> MDETGKELVLALYDYQEKSPREVTM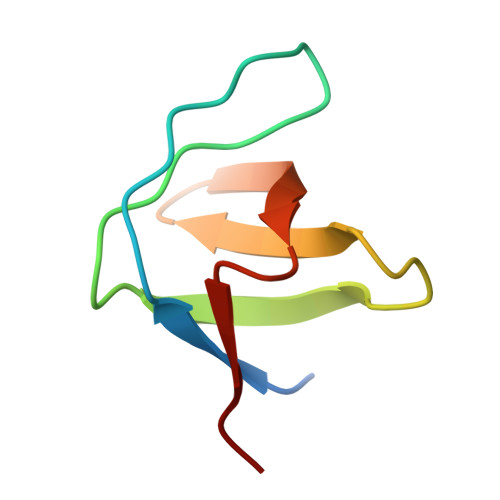KKGDILTLLNSTNKDWWKTEVNGRQGFVPAAYVKKLD Xylitol | C5 H12 O5 | 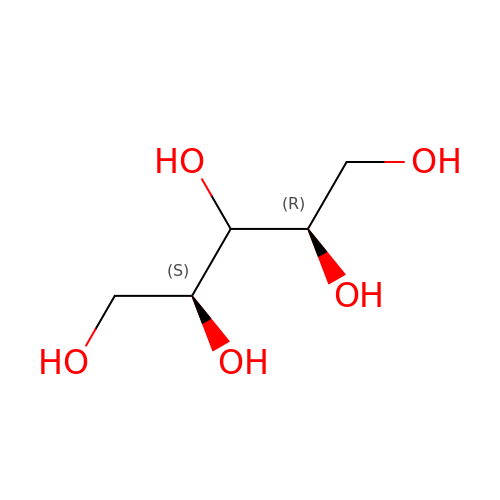HEBKCHPVOIAQTA-SCDXWVJYSA-N The proteins SO_1444 (ParESO) and SO_1445 (CopASO) in the CP4So prophage from Shewanella oneidensis were recently characterized as a typical type II TA pair, with an important role in CP4So maintenance after its excision in host cells. The toxin ParESO can severely inhibit cell growth and cause filamentous growth. The antitoxin CopASO can neutralize ParESO toxicity by direct and tight protein–protein binding. CopASO can bind to a DNA motif in the promoter region containing two inverted repeats (5′-GTANTAC (N)3GTANTAC-3′) to repress the transcription of the TA operon.

The crystal structure of the ParESO-CopASO complex was determined by the single-wavelength anomalous dispersion (SAD) method using a Se-Met-labeled protein. The structure belonged to the space group P43212, and was refined to a final R/Rfree factor of 0.29/0.30 at 3.80 Å resolution. There was a CopASO homodimer binding two respective ParESO molecules in an asymmetric unit (ASU). The resulting heterotetramer adopted an overall very open, V-shaped architecture with the organization of ParESO-(CopASO)2-ParESO. The antitoxin CopASO is composed of an N-terminal RHH domain (β1, α1, and extended α2) and a C-terminal toxin-binding domain (α3 and the extended loop). The two neighboring CopASO molecules dimerize via the RHH domain to mediate the DNA binding. Notably, the intrinsically disordered C-terminal domain is induced to fold into a partially ordered conformation upon ParESO binding. Moreover, the conformations of C-terminal extension in the two CopASO molecules are distinct, and part of the extension is further folded into a helix (α3) in CopASO (I). Structural analysis showed that the toxin–antitoxin contacts were mainly mediated by the C-terminal domain (α3 and C-terminus of α2) of CopASO and the two helices (α1 and α2) of ParESO. Remarkably, surface-charge analysis of CopASO showed the C-terminal extension was predominantly distributed with negative charges (such as Glu54, Glu60, Glu61, and Glu86), which perfectly complemented positively charged regions in and around the binding grooves (such as Arg18, Arg22, and Arg90).

>MSTIKPVSVKLDADIKARVEHLAETRKRSSHWMMREAIREYVEREEKREALQQEALRAWEEHQTSGLHVTGDEVVSWLESWGSENEQAALHATNSLHCHCIT[2x];>[2x]MPQIVFTATALRDLERLREFLRSKNPPAAQRAASAIINTIRKLESYPDIGRPIDDNDFSFRELLIDFGDTGYLAMYQYDGGERLTVLCIRHQKEAGY>MGGFSQSCLPNWIMHGKSCYLFSFSGNSWYGSKRHCSQLGAHLLKIDNSKEFEFIESQTSSHRINAFWIGL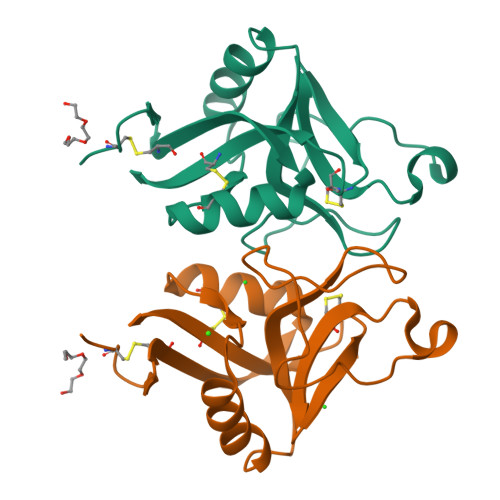SRNQSEGPWFWEDGSAFFPNSFQVRNAVPQESLLHNCVWIHGSEVYNQICNTSSYSICEKELKHHHHHH[2x]>PAGIIPTGNVLSTIEVCAHRCIFDFFKQIRSDDNSLYSAQFDILLGTYCNTLNFVRFLELGLSVACICTKFPELAYVRDGVIQFEVQQPMIARDGPHPVDQPVHNYMVKRIHKRSLSAAFAIASEALSLLSNTYVDGTEIDSSLRIRAIQQMARNLRTVLDSFERGTADQLLGVLLEKAPPLSLLSPINKFQPEGHLNRVARAALLSDLKRRVCADMFFMTRHAREPRLISAYLSDMVSCTQPSVMVSRITHTNTRGRQVDGVLVTTATLKRQLLQGILQIDDTAADVPVTYGEMVLQGTNLVTALVMGKAVRGMDDVARHLLDITDPNTLNIPSIPPQSNSDSTTAGLPVNARVPADLVIVGDKLVFLEALERRVYQATRVAYPLIGNIDITFIMPMGVFQANSMDRYTRHAGDFSTVSEQDPRQFPPQGIFFYNKDGILTQLTLRDAMGTICHSSLLDVEATLVALRQQHLDRQCYFGVYVAEGTEDTLDVQMGRFMETWADMMPHHPHWVNEHLTILQFIAPSNPRLRFELNPAFDFFVAPGDVDLPGPQRPPEAMPTVNATLRIINGNIPVPLCPISFRDCRGTQLGLGRHTMTPATIKAVKDTFEDRAYPTIFYMLEAVIHGNERNFCALLRLLTQCIRGYWEQSHRVAFVNNFHMLMYITTYLGNGELPEVCINIYRDLLQHVRALRQTITDFTIQGEGHNGETSEALNNILTDDTFIAPILWDCDALIYRDEAARDRLPAIRVSGRNGYQALHFVDMAGHNFQRRDNVLIHGRPVRGDTGQAIPITPHHDREWGILSKIYYYIVIPAFSRGSCCTMGVRYDRLYPALQAVIVPEIPADEEAPTTPEDPRHPLHAHQLVPNSLNVYFHNAHLTVDGDALLTLQELMGDMAERTTAILVSSAPDAGAATATTRNMRIYDGALYHGLIMMAYQAYDETIATGTFFYPVPVNPLFACPEHLASLRGMTNARRVLAKMVPPIPPFLGANHHATIRQPVAYHVTHSKSDFNTLTYSLLGGYFKFTPISLTHQLRTGFHPGIAFTVVRQDRFATEQLLYAERASESYFVGQIQVHHHDAIGGVNFTLTQPRAHVDLGVGYTAVCATAALRCPLTDMGNTAQNLFFSRGGVPMLHDNVTESLRRITASGGRLNPTEPLPIFGGLRPATSAGIARGQASVCEFVAMPVSTDLQYFRTACNPRGRASGMLYMGDRDADIEAIMFDHTQSDVAYTDRATLNPWASQKHSYGDRLYNGTYNLTGASPIYSPCFKFFTPAEVNTNCNTLDRLLMEAKAVASQSSTDTEYQFKRPPGSTEMTQDPCGLFQEAYPPLCSSDAAMLRTAHAGETGADEVHLAQYLIRDASPLRGCLPL[5x];> IPAGIIPTGNVLSTIEVCAHRCIFDFFKQIRSDDNSLYSAQFDILLGTYCNTLNFVRFLELGLSVACICTKFPELAYVRDGVIQFEVQQPMIARDGPHPVDQPVHNYMVKRIHKRSLSAAFAIASEALSLLSNTYVDGTEIDSSLRIRAIQQMARNLRTVSDSFERGTADQLLGVLLEKAPPLSLLSPINKFQPEGHLNRVARAALLSDLKRRVCADMFFMTRHAREPRLISAYLSDMVSCTQPSVMVSRITHTNTRGRQVDGVLVTTATLKRQLLQGILQIDDTAADVPVTYGEMVLQGTNLVTALVMGKAVRGMDDVARHLLDITDPNTLNIPSIPPQSNSDSTTAGLPVNARVPADLVIVGDKLVFLEALERRVYQATRVAYPLIGNIDITFIMPMGVFQANSMDRYTRHAGDFSTVSEQDPRQFPPQGIFFYNKDGILTQLTLRDAMGTICHSSLLDVEATLVALRQQHLDRQCYFGVYVAEGTEDTLDVQMGRFMETWADMMPHHPHWVNEHLTILQFIAPSNPRLRFELNPAFDFFVAPGDVDLPGPQRPPEAMPTVNATLRIINGNIPVPLCPISFRDCRGTQLGLGRHTMTPATIKAVKDTFEDRAYPTIFYMLEAVIHGNERNFCALLRLLTQCIRGYWEQSHRVAFVNNFHMLMYITTYLGNGELPEVCINIYRDLLQHVRALRQTITDFTIQGEGHNGETSEALNNILTDDTFIAPILWDCDALIYRDEAARDRLPAIRVSGRNGYQALHFVDMAGHNFQRRDNVLIHGRPVRGDTGQAIPITPHHDREWGILSKIYYYIVIPAFSRGSCCTMGVRYDRLYPALQAVIVPEIPADEEAPTTPEDPRHPLHAHQLVPNSLNVYFHNAHLTVDGDALLTLQELMGDMAERTTAILVSSAPDAGAATATTRNMRIYDGALYHGLIMMAYQAYDETIATGTFFYPVPVNPLFACPEHLASLRGMTNARRVLAKMVPPIPPFLGANHHATIRQPVAYHVTHSKSDFNTLTYSLLGGYFKFTPISLTHQLRTGFHPGIAFTVVRQDRFATEQLLYAERASESYFVGQIQVHHHDAIGGVNFTLTQPRAHVDLGVGYTAVCATAALRCPLTDMGNTAQNLFFSRGGVPMLHDNVTESLRRITASGGRLNPTEPLPIFGGLRPATSAGIARGQASVCEFVAMPVSTDLQYFRTACNPRGRASGMLYMGDRDADIEAIMFDHTQSDVAYTDRATLNPWASQKHSYGDRLYNGTYNLTGASPIYSPCFKFFTPAEVNTNCNTLDRLLMEAKAVASQSSTDTEYQFKRPPGSTEMTQDPCGLFQEAYPPLCSSDAAMLRTAHAGETGADEVHLAQYLIRDASPLRGCLPL;> NIPAGIIPTGNVLSTIEVCAHRCIFDFFKQIRSDDNSLYSAQFDILLGTYCNTLNFVRFLELGLSVACICTKFPELAYVRDGVIQFEVQQPMIARDGPHPVDQPVHNYMVKRIHKRSLSAAFAIASEALSLLSNTYVDGTEIDSSLRIRAIQQMARNLRTVSDSFERGTADQLLGVLLEKAPPLSLLSPINKFQPEGHLNRVARAALLSDLKRRVCADMFFMTRHAREPRLISAYLSDMVSCTQPSVMVSRITHTNTRGRQVDGVLVTTATLKRQLLQGILQIDDTAADVPVTYGEMVLQGTNLVTALVMGKAVRGMDDVARHLLDITDPNTLNIPSIPPQSNSDSTTAGLPVNARVPADLVIVGDKLVFLEALERRVYQATRVAYPLIGNIDITFIMPMGVFQANSMDRYTRHAGDFSTVSEQDPRQFPPQGIFFYNKDGILTQLTLRDAMGTICHSSLLDVEATLVALRQQHLDRQCYFGVYVAEGTEDTLDVQMGRFMETWADMMPHHPHWVNEHLTILQFIAPSNPRLRFELNPAFDFFVAPGDVDLPGPQRPPEAMPTVNATLRIINGNIPVPLCPISFRDCRGTQLGLGRHTMTPATIKAVKDTFEDRAYPTIFYMLEAVIHGNERNFCALLRLLTQCIRGYWEQSHRVAFVNNFHMLMYITTYLGNGELPEVCINIYRDLLQHVRALRQTITDFTIQGEGHNGETSEALNNILTDDTFIAPILWDCDALIYRDEAARDRLPAIRVSGRNGYQALHFVDMAGHNFQRRDNVLIHGRPVRGDTGQAIPITPHHDREWGILSKIYYYIVIPAFSRGSCCTMGVRYDRLYPALQAVIVPEIPADEEAPTTPEDPRHPLHAHQLVPNSLNVYFHNAHLTVDGDALLTLQELMGDMAERTTAILVSSAPDAGAATATTRNMRIYDGALYHGLIMMAYQAYDETIATGTFFYPVPVNPLFACPEHLASLRGMTNARRVLAKMVPPIPPFLGANHHATIRQPVAYHVTHSKSDFNTLTYSLLGGYFKFTPISLTHQLRTGFHPGIAFTVVRQDRFATEQLLYAERASESYFVGQIQVHHHDAIGGVNFTLTQPRAHVDLGVGYTAVCATAALRCPLTDMGNTAQNLFFSRGGVPMLHDNVTESLRRITASGGRLNPTEPLPIFGGLRPATSAGIARGQASVCEFVAMPVSTDLQYFRTACNPRGRASGMLYMGDRDADIEAIMFDHTQSDVAYTDRATLNPWASQKHSYGDRLYNGTYNLTGASPIYSPCFKFFTPAEVNTNCNTLDRLLMEAKAVASQSSTDTEYQFKRPPGSTEMTQDPCGLFQEAYPPLCSSDAAMLRTAHAGETGADEVHLAQYLIRDASPLRGCLPL;>[6x]SNPTTFSVEAIAAYTPVALIRLLNASGPLQPGHRVDIADARSIYTVGAAASAARARANHNANTIRRTAMFAETDPMTWLRPTVGLRRTFNPRII;>[2x]AMPFEIEVLLPGELSPAETSALQKCEGKIITFSTLRHRASLVDIALSSYYINGAPPDTLSLLEAYRMRFAAVITRVIPGKLLAHAIGVGTPTPGLFIQNTSPVDLCNGDYICLLPPVYGSADSIRLDSVGLEIVFPLTIPQTLMREIIAKVVARAVEDLNLMFSINEGCLLILALIPRLLALLIPRLLALVTREAAQLIHPEAPMLMLPIYETISSWISTSSRLGDTLGTRAILRVCVFDGPSTVHPGDRTAVIQV;>[2x]AMPFEIEVLLPGEISPAETSALQKCEGKIITFSTLRHRASLVDIALSSYYINGAPPDTLSLLEAYRMRFAAVITRVIPGKLLAHAIGVGTPTPGLFIQNTSPVDLCNGDYICLLPPVFGSADEIRLDSVGLEIVFPLTIPQTLMREIIAKVVARAVERTAADVICYNGRRYELETNLQHRDGSDAAIRTLVLNLMFSINEGTTLILTLITRLLRFPIYEAISSWISTSSRLGDTLGTRAILRVCVFDGPSTVHPGDRTAVIQV;>[2x]FKSTTQLIQQVSLTDFFRPDIEHAGSTVLILRHPTDLPALARHRAPPGRQTERLAEAWGQLLEASRAYVTSLSFIAACRAEEYTDKQAAEANRTAIVSAYGCSRMGARLIRFSECLRAMVQCHVFPHRFISFFGSLLEYTIQDNLCNITAVAKGPQEAARTDKTSTRRVTANIPACVFWDVDKDLHLSADGLKHVFLVFVYTQRRQREGVRLHLALSQLNEQCFGRGIGFLLGARICMYAAYTLIGTIPSESVRYTRRMERFGGYNVPTIWLEGVVWGGTNTWNEC;> MNAHLANEVQYDLGHPSSLVHVIISSECLAAAGIPLAALMRANFQVEIQTRAHATGDCTPWCTAFAAYVPADAVGELLAPVVPAHPGLLPRASSAGGLFVSLPVVCDAQGVYDPYAVAALRLAWGSGASCARVILFSYDELVPPNTRYAADSTRIMRVCRHLCRYVALLGAAAPPAAKEAAAHLSMGLPPISPEEQLTAPGGDTTAAQDVSIAQENEEILALVQRRSLVEWLDRGWEALAGGDRPDWLWSRRSISVVLRHHYGTKQRFVVVSYENSVAWGGRRARPPLLSSALATALTEACAAERVVRPHQLSPAGQAELLLRFPALEVPLRHPRPVLPPFDIAAEVAFTARIHLACLRALGQAIRAA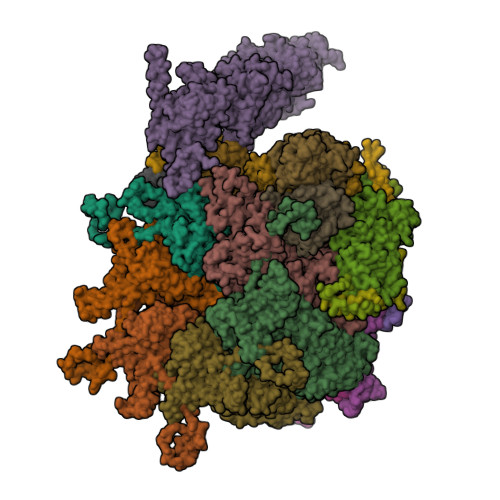LQGGPRISQRLRYDFGPDQRAWLGEVTRRFPILLENLMRAVEGTAPDAFFHTAYALAVLAHLGGRVVPLGDDLPARFADSDGHYVFDYYSTSGDTLRLNNRPIAVAMDEQSKCRFMEAPRRVCEQYLPGESYAYLCLGFNRRLCGIVVFPGGFAFTINIAAYLSLSDPVARAAVLRFCRKVS;> MDPYCPFDALDVWEHRRFIVADSRNFITPEFPRDFWMSPVFNLPRETAAEQVVVLQAQRTAAAAALENAAMQAAELPVDIERRLRPIERNVHEI;> WEHRRFIVADSRNFITPEFPRDFWMSPVFNLPRETAAEQVVVLQAQRTAAAAALENAAMQAAELPVDIERRLRPIERNVH;>QRTGRSALAVLIRACYRLQQQLQRTRRALLHHSDAVLTSLHHVRMLL[2x]> SSQIRQNYSTEVEAAVNRLVNLYLRASYTYLSLGFYFDRDDVALEGVCHFFRELAEEKREGAERLLKMQNQRGGRALFQDLQKPSQDEWG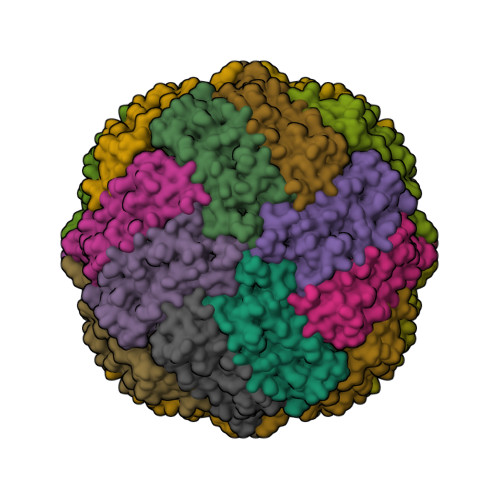TTLDAMKAAIVLEKSLNQALLDLAALGSAQADPHLCDFLESHFLDEEVKLIKKMGDHLTNIQRLVGSQAGLGEYLFERLTLKHD> TSSKIYDNKNQLIADL;> NYPAYMDNYLKEVINQVEEETGYNLLTTGMDVYTNVDQEAQKHLWDIYNTDEYVAYPDDELQV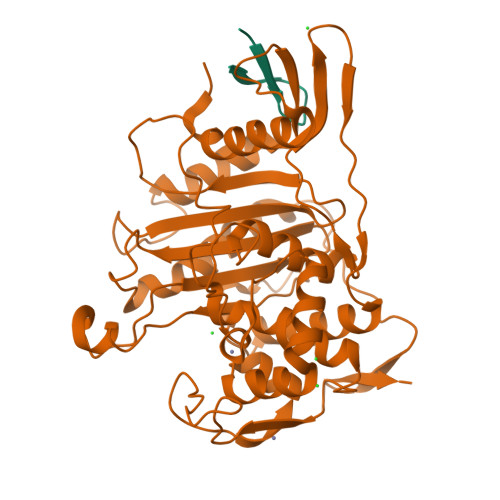ASTIVDVSNGKVIAQLGARHQSSNVSFGINQAVETNRDWGSTMKPITDYAPALEYGVYDSTATIVHDEPYNYPGTNTPVYNWDRGYFGNITLQYALQQSRNVPAVETLNKVGLNRAKTFLNGLGIDYPSIHYSNAISSNTTESDKKYGASSEKMAAAYAAFANGGTYYKPMYIHKVVFSDGSEKEFSNVGTRAMKETTAYMMTDMMKTVLTYGTGRNAYLAWLPQAGKTGTSNYTDEEIENHIKTSQFVAPDELFAGYTRKYSMAVWTGYSNRLTPLVGNGLTVAAKVYRSMMTYLSEGSNPEDWNIPEGLYRNGEFVFKN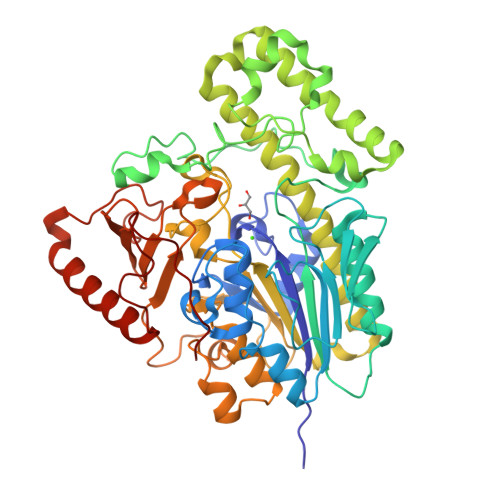>[2x]QTKAEENKKPNILFIITDDHAYQTLGTGNNDSPVALPNFNKLGRQGMVFDRSYCANSLCGPSRACILTGRHSHMNGFVFNGQRPLDGSQPTYPKMLQKAGYQTGLFGKWHLESDPTGFDTWEIFPGQGSYYNPDFISLKPDGKRQTKRFPGYATDVVTDKSIQWLGNRDKNKPFLLVVGHKAPHRAWCPALRHLGKVDTSSMTPPANFHDDYANRPEFLKKNQQTVANHMAIYSDLKVLKDQVPEEMRKSIVSPGYGWDLGELNRMTPEEKKTWTDYYAKRTKSLVDGMKSGKLKDPKAFAEWKWHAYMEDYLGCLLSVDDSIGRLMEYLDKEGIAKDTLVIYCGDQGFYMGEHGMYDKRWIFEESLRMPLIMRWPGKIPAGIRNNTMVQNIDYAPTIVSAAGADTPENMNTFQGVSLLPTAFTGKTPDNWRDAIYYCFYENPGEHNAPRHDGIRTDRYTLSYIWTSDEWMLFDMKKDPMQMKNVIDDPAYKTTVEQLKKRYHELRKTYKVPENSPGGKGTPIPKFDASW3-[[4-oxidanyl-1-[(3~{R})-3-phenylbutanoyl]piperidin-4-yl]methyl]-6-(2-pyrrolidin-1-ylethylamino)pyrimidin-4-one | C26 H37 N5 O3 | 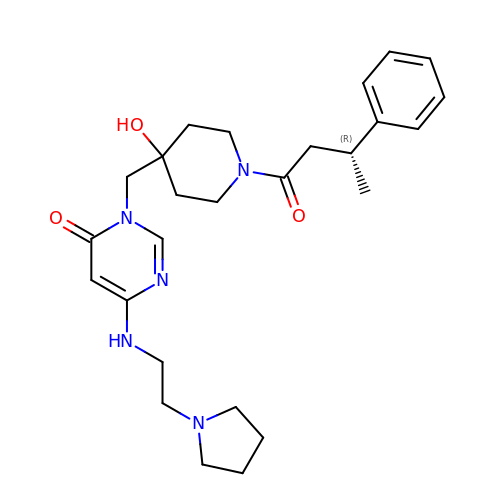VJDZJAUBPMXVAF-OAQYLSRUSA-N>CGUGAUCGC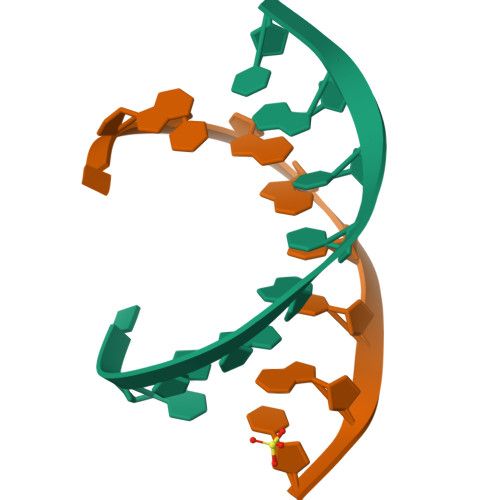[2x]>GHMAKKKATETTDEDEDGGSEKKYRKCEKAGCTATCPVCFASASERCAKNGYTSRWYHLSCGEHFCNECFDHYYRSHKDGYDKYTTWKKIWTSNGKTEPSPKAFMADQQLPYWVQCTKPECRKWRQLTKEIQLTPQIAKTYRCGMKPNTAIKPETSDHCSLPEDLRVLEVSNHWWYSMLILPPLLKDSVAAPLLSAYYPDCVGMSPSCTSTNRAAATGNASPGKLEHSKAALSVHVPGMNRYFQPFYQPNECGKALCVRPDVMELDELYEFPEYSRDPTMYLALRNLILALWYTNCKEALTPQKCIPHIIVRGL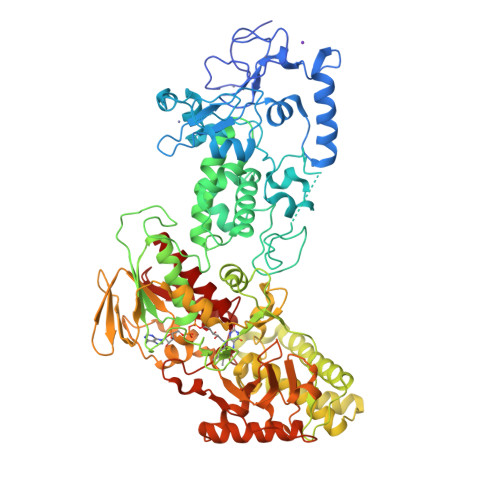VRIRCVQEVERILYFMTRKGLINTGVLSVGADQYLLPKDYHNKSVIIIGAGPAGLAAARQLHNFGIKVTVLEAKDRIGGRVWDDKSFKGVTVGRGAQIVNGCINNPVALMCEQLGISMHKFGERCDLIQEGGRITDPTIDKRMDFHFNALLDVVSEWRKDKTQLQDVPLGEKIEEIYKAFIKESGIQFSELEGQVLQFHLSNLEYACGSNLHQVSARSWDHNEFFAQFAGDHTLLTPGYSVIIEKLAEGLDIQLKSPVQCIDYSGDEVQVTTTDGTGYSAQKVLVTVPLALLQKGAIQFNPPLSEKKMKAINSLGAGIIEKIALQFPYRFWDSKVQGADFFGHVPPSASKRGLFAVFYDMDPQKKHSVLMSVIAGEAVASVRTLDDKQVLQQCMATLRELFKEQEVPDPTKYFVTRWSTDPWIQMAYSFVKTGGSGEAYDIIAEDIQGTVFFAGEATNRHFPQTVTGAYLSGVREASKIAAF[2x]> MVYSYTEKKRIRKDFGKRPQVLDVPYLLSIQLDSFQKFIEQDPEGQYGLEAAFRSVFPIQSYSGNSELQYVSYRLGEPVFDVQECQIRGVTYSAPLRVKLRLVIYEREAPEGTVKDIKEQEVYMGEIPLMTDNGTFVINGTERVIVSQLHRSPGVFFDSDKGKTHSSGKVLYNARIIPYRGSWLDFEFDPKDNLFVRIDRRRKLPATIILRALNYTTEQILDLFFEKVIFEIRDNKLQMELVPERLRGETASFDIEANGKVYVEKGRRITARHIRQLEKDDVKLIEVPVEYIAGKVVAKDYIDESTGELICAANMELSLDLLAKLSQSGHKRIETLFTNDLDHGPYISETLRVDPTNDRLSALVEIYRMMRPGEPPTREAAESLFENLFFSEDRYDLSAVGRMKFNRSLLREEIEGSGILSKDDIIDVMKKLIDIRNGKGEVDDIDHLGNRRIRSVGEMAENQFRVGLVRVERAVKERLSLGDLDTLMPQDMINAKPISAAVKEFFGSSQLSQFMDQNNPLSEITHKRRILALGPGGLTRERAGFEVRDVHPTHYGRVCPI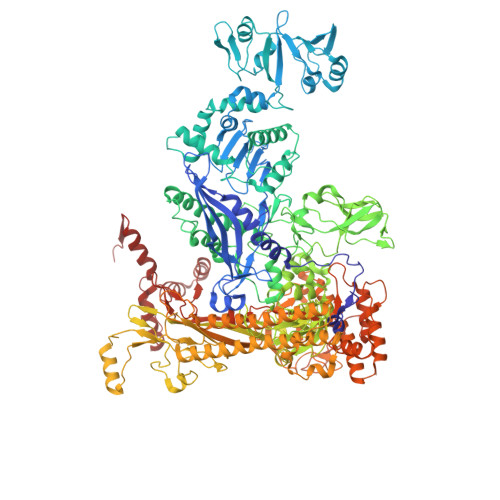ETPEGPNIGLINSLSVYAQTNEYGFLETPYRKVTDGVVTDEIHYLSAIEEGNYVIAQANSNLDEEGHFVEDLVTCRSKGESSLFSRDQVDYMDVSTQQVVSVGASLIPFLEHDDANRALMGANMQRQAVPTLRADKPLVGTGMERAVAVDSGVTAVAKRGGVVQYVDASRIVIKVNEDEMYPGEAGIDIYNLTKYTRSNQNTCINQMPCVSLGEPVERGDVLADGPSTDLGELALGQNMRVAFMPWNGYNFEDSILVSERVVQEDRFTTIHIQELACVSRDTKLGPEEITADIPNVGEAALSKLDESGIVYIGAEVTGGDILVGKVTPKGETQLTPEEKLLRAIFGEKASDVKDSSLRVPNGVSGTVIDVQVFTRDGVEKDKRALEIEEMQLKQAKKDLSEELQILEAGLFSRIRAVLVAGGVEAEKLDKLPRDRWLELGLTDEEKQNQLEQLAEQYDELKHEFEKKLEAKRRKITQGDDLAPGVLKIVKVYLAVKRRIQPGDKMAGRHGNKGVISKINPIEDMPYDENGTPVDIVLNPLGVPSRMNIGQILETHLGMAAKGIGDKINAMLKQQQEVAKLREFIQRAYDLGADVRQKVDLSTFSDEEVMRLAENLRKGMPIATPVFDGAKEAEIKELLKLGDLPTSGQIRLYDGRTGEQFERPVTVGYMYMLKLNHLVDDKMHARSTGSYSLVTQQPLGGKAQFGGQRFGEMEVWALEAYGAAYTLQEMLTVKSDDVNGRTKMYKNIVDGNHQMEPGMPESFNVLLKEIRSLGINIELEDE> MAHTAAERPPEETLSLWKGEQARLKARVVDRDTEAWQRDPSFSGLQKVGGVAVSFVKGDSVRACASLVVLSYPELKVVYEDSRMVGLKAPYVSGFLAFREVPFLVELVQRLQEKEPDLMPQVVLVDGNGVLHQRGFGVACHLGVLTELPCIGVAKKLLQVDGLENNALHKEKIVLLQAGGDTFPLIGSSGTVLGMALRSHDHSTKPLYVSVGHRISLEVAVRLTHHCCRFRIPEPIRQADIRSREYIRRT

Removal of inosines from genomic DNA is dealt with by the base excision repair pathway as well as endonuclease V (EndoV), which is considered the major player. The mouse genome encodes a single EndoV homolog, mEndoV. Our data show that mEndoV shares substrate preferences with hEndoV by catalyzing cleavage at inosines in RNA and being inert towards inosines in DNA. The structure determination of mEndoV revealed a protein fold which is to a large extent similar to human and prokaryotic EndoVs.

The first 9 residues on the N-terminal end are disordered with no specific conformation. The region around residues 167–174 contains a mammalian specific α-helix similar to that of hEndoV. The structure of mouse EndoV reveals a new conformation of the highly conserved strand-separating wedge motif. The invariant Tyr residue, normally pointing into the DNA/RNA binding groove and stacking with the DNA/RNA substrate during catalysis, is facing away from the groove. For this reason, the DNA/RNA binding groove in the crystal structure of mouse EndoV in the unbound state is wide and shallow. In contrast to all other reported EndoV structures, the invariant Tyr91 in mEndoV is interacting with the backbone of the protein through hydrogen bonds to Ser60, Val61 and Leu87. In order to stack with nucleotides in the active site pocket, the mEndoV Tyr91 must undergo a transition to the trans side chain conformation for χ1. The MD simulation suggests that the wedge motif has some flexibility and that the invariant Tyr might flip between two conformations, of which a probably unbound or unproductive state is shown in the structure of mEndoV. The corresponding region in mEndoV is 225-HHCC-228, and our structure of mEndoV reveals that the first two Cys residues in hEndoV are replaced by histidines with no change in the local geometry. The latter two Cys residues are conserved between mouse and human EndoV, and with similar conformations and local environment in the two structures.>AVYTLPELPYDYSALEPYISGEIMELHHDKHHKAYVDGANTALDKLAEARDKADFGAINKLEKDLAFNLAGHVNHSVFWKNMAPKGSAPERPTDELGAAIDEFFGSFDNMKAQFTAAATGIQGSGWASLVWDPLGKRINTLQFYDHQNNLPAGSIPLLQLDMWEHAFYLQYKNVKGDYVKSWWNVVNWDDVALRFSEARVA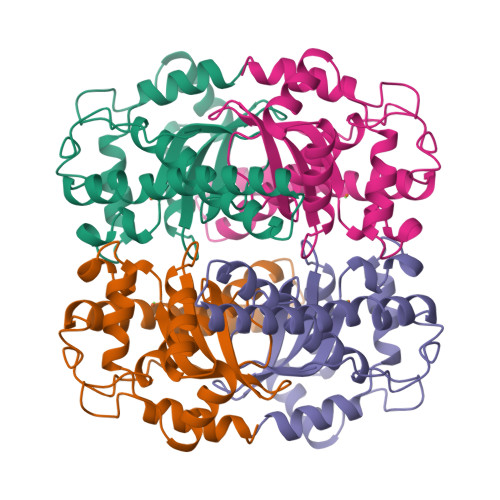[2x]There are two major types of galactolipids in chloroplastic membranes: monogalactosyldiacylglycerol and digalactosyldiacylglycerol (DGDG). A major percentage of MGDG is further galactosylated to DGDG, a process that is catalyzed by digalactosyldiacylglycerol synthases. However, during phosphate shortage, DGD2 is upregulated and synthesizes DGDG in the outer membrane of the chloroplast. Herein, we present the X-ray crystal structure of the integral monotropic membrane protein atDGD2, bound to its donor nucleotide-sugar substrate UDP-galactose.

The X-ray crystal structure of atDGD2 in complex with its substrate UDP-galactose was solved in space group P41212 to 2.10 Å resolution. The protein crystallizes as a monomer in the asymmetric unit. The atDGD2 monomer has a classic GT-B fold, comprised of two distinct Rossmann-like β/α/β domains connected by a flexible loop region. The nucleotide sugar binds in a deep cleft between the individual N- and C-terminal domains. The atDGD2 structure showed clear electron density for UDP-galactose, which binds the enzyme in the anti glycosidic conformation. The ligand is positioned by residues from both the N- and C-terminal domains of the protein. However, there were four residues (Gly22, His151, Lys243, and Glu321, atDGD2 numbering) which were shown to be entirely conserved between the structures. These residues are important for positioning either the ribose (Glu321), phosphate group (Gly22 and Lys243), or galactose (His151) moieties of atDGD2. In the N-terminal domain there are two areas of missing electron density corresponding to residues 133 to 137 and 163 to 169. B-factor analysis shows that the areas around the missing density in atDGD2 have the highest temperature factors in the structure, which suggests that the absence of electron density is a result of structural flexibility.

> MTNQQEQHIAIFTTASIPWLTGTAVNPLFRAAYLANDGERRVTLVIPWLTLKHQKLVYPNSITFSSPSEQEAYVRQWLEERVSFRLAFEIRFYPGKFAIDKRSILPVGDISDAIPDEEADIAVLEEPEHLTWFHHGQKWKTKFNYVIGIVHTNYLEYVKREKQGRVKAFFLKYLNSWVVGIYCHKVIRLSAATQEYPKSIVCNVHGVNPKFLEIGLRKLEQQKLQEQPFTKGAYYIGKMVWSKGYKELLKLLEKHQKELAELEVDLYGDGEDSEEIKEAARKLDLTVNVYPGRDHADSLFHNYKVFLNPSTTDVVCTTTAEALAMGKIVVCANHISNKFFKQFPNCRTYDDGQGFVRATLKALGEQPSQLTEQQRHELSWEAATQRFIKVSDLNRLSRADKLAAHHHHHHHH>[2x]MGHHHHHHSSYTSITKLTNLTEFRNLIKQNDKLVIDFYATWCGPCKMMQPHL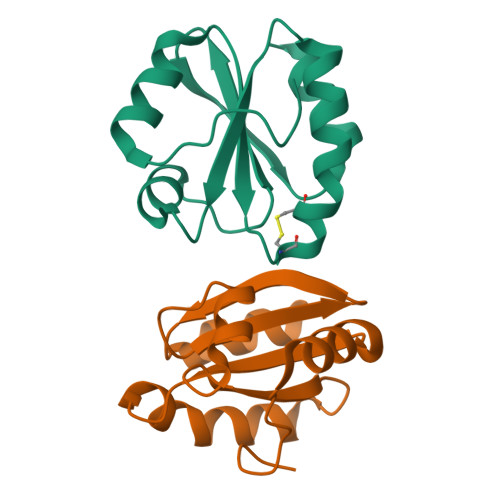TKLIQAYPDVRFVKCDVDESPDIAKECEVTAMPTFVLGKDGQLIGKIIGANPTALEKGIKDL> MGSWSHPQFEKGMVTKKAKVYKKASPNGKLTTYLAKRDYYDHKEWQDNIDGVCVVDPDYLKNRKVFGLIVVAFRYGREDMDVMGVSF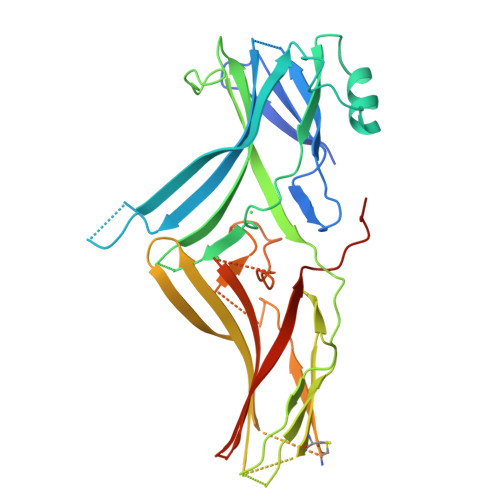RKDFAVKQMQIYPPLEENQRPLTKLQAKLLNKLGENAVPFHYDLPTNTPDTVCIQPSEYDGGAPCGVDYQVTTYVSQNMDDKIHKRNSVSLSIRKLSYFEFGSDEQPRGEISKEFKFTSGAMKLECTLDKARYYSGESMNISVCVDNPTSKKAKRIKIQIIQLADICLYETVTYKSVVTELETEEGFPIEPNTSGFCQVYKLRPVLEVTKRRAGLALNGKVKYEDTMLAASTEDAGNVDKENLGVVVSYKVRIKMTLGFGSGDMLLEVPFKLCPARLKGRLAQPEAREGDDAE> MGCDRNCGLIAGAVIGAVLAVFGGILMPVGDLLIQKTIKKQVVLEEGTIAFKNWVKTGTEVYRQFWIFDVQNPQEVMMNSSNIQVKQRGPYTYRVRFLAKENVTQDAEDNTVSFLQPNGAIFEPSLSVGTEADNFTVLNLAVAAASHIYQNQFVQMILNSLINKSKSSMFQVRTLRELLWGYRDPFLSLVPYPVTTTVGLFYPYNNTADGVYKVFNGKDNISKVAIIDTYKGKRNLSYWESHCDMINGTDAASFPPFVEKSQVLQFFSSDICR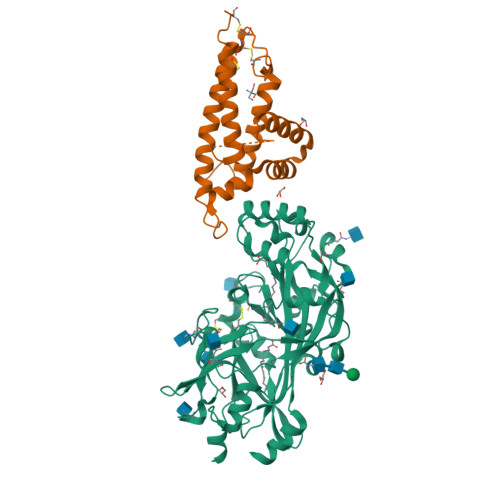SIYAVFESDVNLKGIPVYRFVLPSKAFASPVENPDNYCFCTEKIISKNCTSYGVLDISKCKEGRPVYISLPHFLYASPDVSEPIDGLNPNEEEHRTYLDIEPITGFTLQFAKRLQVNLLVKPSEKIQVLKNLKRNYIVPILWLNETGTIGDEKANMFRSQVTGKINLLGLIEMILLSVGVVMFVAFMISYCACRSKTIK;> EDKIMSYNAFFWMWVHDMLIDSIKWRDEHGRCINKDKGKTCIKGCNKKCISFQKWVEQKKTEWGKIKDHFRKQKDIPKDWTHDDFLQTLLMKDLLLEIIQDTYGDANEIKRIEALLEQAGVGGIDFAALAGLYTKGFVAEKDTTIDKLLQHEQKEADKCLKTHTDDTCPPQEDRSVARS>[2x]DDNGIVLLGERAAKCRAYAKALHYKELEFQKGPTPAILESLISINNKLQQPEAAAGVLEYAMKHFGELEIQATWYEKLHEWEDALVAYDKKMDTNKDDPELMLGRMRCLEALGEWGQLHQQCCEKWTLVNDETQAKMARMAAAAAWGLGQWDSMEEYTCMIPRDTHDGAFYRAVLALHQDLFSLAQQCIDKARDLLDAELTAMAGESYSRAYGAMVSCHMLSELEEVIQYKLVPERREIIRQIWWERLQGCQRIVEDWQKILMVRSLVVSPHEDMRTWLKYASLCGKSGRLALAHKTLVLLLGVDPSRQLDHPLPTVHPQVTYAYMKNMWKSARKIDAFQHMQHFVQTMQQQAQHAIATEDQQHKQELHKLMARCFLKLGEWQLNLQGINESTIPKVLQYYSAATEHDRSWYKAWHAWAVMNFEAVLHYKHQNQARDEKKKLRHASGANITNATTAATTAATATTTASTEGSNSESEAESTENSPTPSPLQKKVTEDLSKTLLMYTVP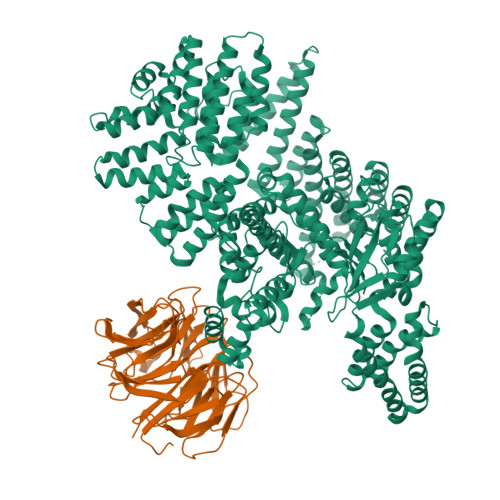AVQGFFRSISLSRGNNLQDTLRVLTLWFDYGHWPDVNEALVEGVKAIQIDTWLQVIPQLIARIDTPRPLVGRLIHQLLTDIGRYHPQALIYPLTVASKSTTTARHNAANKILKNMCEHSNTLVQQAMMVSEELIRVAILWHEMWHEGLEEASRLYFGERNVKGMFEVLEPLHAMMERGPQTLKETSFNQAYGRDLMEAQEWCRKYMKSGNVKDLTQAWDLYYHVFRRISKQLPQLTSLELQYVSPKLLMCRDLELAVPGTYDPNQPIIRIQSIAPSLQVITSKQRPRKLTLMGSNGHEFVFLLKGHEDLRQDERVMQLFGLVNTLLANDPTSLRKNLSIQRYAVIPLSTNSGLIGWVPHCDTLHALIRDYREKKKILLNIEHRIMLRMAPDYDHLTLMQKVEVFEHAVNNTAGDDLAKLLWLKSPSSEVWFDRRTNYTRSLAVMSMVGYILGLGDRHPSNLMLDRLSGKILHIDFGDCFEVAMTREKFPEKIPFRLTRMLTNAMEVTGLDGNYRITCHTVMEVLREHKDSVMAVLEAFVYDPLLNWRLMDTNTKGNKRSRTRTDSYSAGQSVEILDGVELGEPAHKKTGTTVPESIHSFIGDGLVKPEALNKKAIQIINRVRDKLTGRDFSHDDTLDVPTQVELLIKQATSHENLCQCYIGWCPFW;>[2x]MNTSPGTVGSDPVILATAGYDHTVRFWQAHSGICTRTVQHQDSQVNALEVTPDRSMIAAAGYQHIRMYDLNSNNPNPIISYDGVNKNIASVGFHEDGRWMYTGGEDCTARIWDLRSRNLQCQRIFQVNAPINCVCLHPNQAELIVGDQSGAIHIWDLKTDHNEQLIPEPEVSITSAHIDPDASYMAAVNSTGNCYVWNLTGGIGDEVTQLIPKTKIPAHTRYALQCRFSPDSTLLATCSADQTCKIWRTSNFSLMTELSIKSGNPGESSRGWMWGCAFSGDSQYIVTASSDNLARLWCVETGEIKREYGGHQKAVVCLAFNDSVLG(2S)-1-(butanoyloxy)-3-{[(R)-hydroxy{[(1S,2R,3R,4R,5R,6S)-2,3,4,5,6-pentahydroxycyclohexyl]oxy}phosphoryl]oxy}propan-2-yl tridecanoate | C26 H49 O13 P | 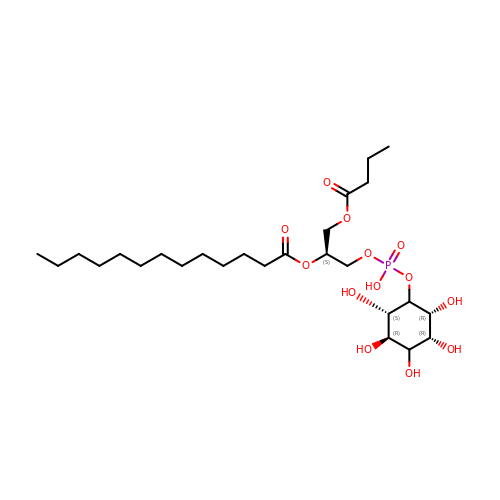PJDJYKJPFGJDMA-STSOKTRESA-N> YSIEADKKFKYSVKLSDYPTLQDAASAAVDGLLIDRDYNFYGGETVDFGGKVLTIECKAKFIGDGNLIFTKLGKGSRIAGVFMESTTTPWVIKPWTDDNQWLTDAAAVVATLKQSKTDGYQPTVSDYVKFPGIETLLPPNAKGQNITSTLEIRECIGVEVHRASGLMAGFLFRGCHFCKMVDANNPSGGKDGIITFENLSGDWGKGNYVIGGRTSYGSASSAQFLRNNGGFERDGGVIGFTSYRAGESGVKTWQGTVGSTTSRNYNLQFRDSVVIYPVWDGFDLGADTDMNPELDRPGDYPITQYPLHQ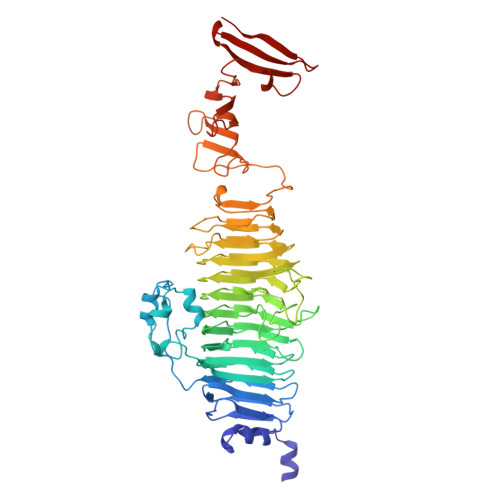LPLNHLIDNLLVRGALGVGFGMDGKGMYVSNITVEDCAGSGAYLLTHESVFTNIAIIDTNTKDFQANQIYISGACRVNGLRLIGIRSTDGQGLTIDAPNSTVSGITGMVDPSRINVANLAEEGLGNIRANSFGYDSAAIKLRIHKLSKTLDSGALYSHINGGAGSGSAYTQLTAISGSTPDAVSLKVNHKDCRGAEIPFVPDIASDDFIKDSSCFLPYWENNSTSLKALVKKPNGELVRLTLATL>LLSGKLTPAQSKNPAKNELYLVEGDSAGGSAKQGRDRKFQAILPLRGKVINTAKAKMADILKNEEINTMIYTIGAGVGADFSIEDANYDKIIIMTDADTDGAHIQTLLLTFFYRYMRPLVEAGHVYIALPPLYKMSKGKGKKEEVAYAWTDGELEELRKQFGKGATLQRYKGLGEMNADQLWETTMNPETRTLIRVTIEDLARAERRVNVLMGDKVEPRRKWIEDNVKFTLEEATVFHMSNIQNMSLEDIMGERFGRYSKYIIQDRALPDIRDGLKPVQRRILYSMNKDSNTFDKSYRKSAKSVGNIMGNFHPHGDSSIYDAMVRMSQNWKNREILVEMHGNNGSMDGDPPAAMRYTEARLSEIAGYLLQDIEKKTVPFAWNFDDTEKEPTVLPAAFPNLLVNGSTGISAGYATDIPPHNLAEVIDAAVYMIDHPTAKIDKLMEFLPGPDFPTGAIIQGRDEIKKAYETGKGRVVVRSKTEIEKLKGGKEQIVITEIPYEINKANLVKKIDDVRVNNKVAGIAEVRDESDRDGLRIAIELKKDANTELVLNYLFKYTDLQINYNFNMVAIDNFTPRQVGIVPILSSYIAHRREVILARSRFDKEKAEKRLHIVEGLIRVISILDEVIALIRASENKADAKENLKVSYDFTEEQAEAIVTLQLYRLTNTDVVVLQEEEAELREKIAMLAAIIGDERTMYNLMKKELREVKKKFATPRLSSLEDT[2x]

Type II topoisomerases (top2) regulate DNA topology which requires divalent metal ions (usually Mg2+) for their enzymatic activity. Metal ions are also known to be essential for fluoroquinolone action in bacterial top2, including gyrase and topoisomerase (topo) IV, which are heterodimers in their active form. Fluoroquinolones act by stabilizing the enzymes in a DNA-cleaved state and subsequently causing bacterial cell death.

S. pneumoniae topo IV ParE30-ParC55 was cocrystalized with an 18 bp dsDNA, stabilized by a fluoroquinolone delafloxacin. Using this instrument, we are able to pinpoint the location of Mg2+ ions in the fluoroquinolone (delafloxacin)-stabilized Streptococcus pneumoniae topo IV cleavage complex with high confidence. One pair of Mg2+ ions (one in each asymmetric ParE–ParC subunit) is bound to each of the two delafloxacin molecules that is hemiintercalated into each DNA strand. Although the full octahedral coordination was not observed in this relatively low-resolution structure, this Mg2+ pair is believed to coordinate the fluoroquinolone molecule through water–ion bridges with a serine (S79) and a downstream acidic residue (D83) that are conserved across bacterial species. The second pair of Mg2+ ions is found at each catalytic pocket of the ParE TOPRIM domain coordinated by the aspartate residues D506 and D508, which correspond to the proposed B-site. This is consistent with the observation of a single catalytic metal at B-site in many other drug-stabilized topo complex structures, which is likely representative of the involvement of Mg2+ in stabilizing the DNA-cleaved conformation. We identified two pairs of K+ ions (one in each asymmetric ParE–ParC subunit). The K+ site is remarkably conserved especially in topo IV of Gram positives suggesting a subunit-bridging role in these enzymes, though divergence of M101 (to G) and N105 (to W/F) in other bacterial top2 might affect K+ binding and enzyme function. A second pair of K+ ions is located in the ParC tower domain coordinating between F316 and N324 (FKYTDLQ), specifically F316, K317, T319, and Q322 and further coordinated through water networks to D320 and N324. Although Cl− are not typically associated with topos, we identified a pair of Cl− ions coordinating between ParE C-terminal residues E609-D610 and ParC N-terminal residues L9-E10, potentially supporting additional structural integrity.>MSAKAISEQTGKELLYKFISTTSAIQNRFKYARVTPDTDWARLLQDHPWLLSQNLVVKPDQLIKRRGKLGLVGVNLTLDGVKSWLKPRLGQEATVGKATGFLKNFLIEPFVPHSQAEEFYVCIYATREGDYVLFHHEGGVDVGDVDAKAQKLLVGVDEKLNPEDIKKHLLVHAPEDKKEILASFISGLFNFYEDLYFTYLEINPLVVTKDGVYVLDLAAKVDATADYICKVKWGDIEFPPPFGREAYPEEAYIADLDAKSGASLKLTLLNPKGRIWTMVAGGGASVVYSDTIGDLGGVNELANYGEYSGAPSEQQTYDYAKTILSLMTREKHPDGKILIIGGSIANFTNVAATFKGIVRAIRDYQGPLKEHEVTIFVRRGGPNYQEGLRVMGEVGKTTGIPIHVFGTETHMTAIVGMALGHRPIPNQPPTAAHTANFLLNASGSTSTPAPSRTASFSESRADEVAPAKKAKPAMPQDSVPSPRSLQGKSTTLFSRHTKAIVWGMQTRAVQGMLDFDYVCSRDEPSVAAMVYPFTGDHKQKFYWGHKEILIPVFKNMADAMRKHPEVDVLINFASLRSAYDSTMETMNYAQIRTIAIIAEGIPEALTRKLIKKADQKGVTII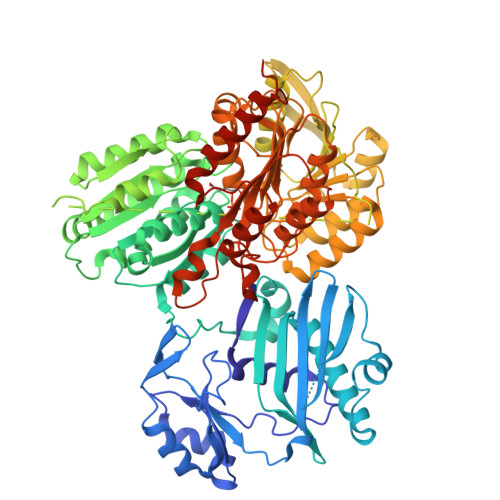GPATVGGIKPGCFKIGNTGGMLDNILASKLYRPGSVAYVSRSGGMSNELNNIISRTTDGVYEGVAIGGDRYPGSTFMDHVLRYQDTPGVKMIVVLGEIGGTEEYKICRGIKEGRLTKPIVCWCIGTCATMFSSEVQFGHAGACANQASETAVAKNQALKEAGVFVPRSFDELGEIIQSVYEDLVANGVIVPAQEVPAALEHHHHHHH[2x]(5-methyl-2-pyridin-4-yl-phenyl)-[4-oxidanyl-4-(phenylmethyl)piperidin-1-yl]methanone 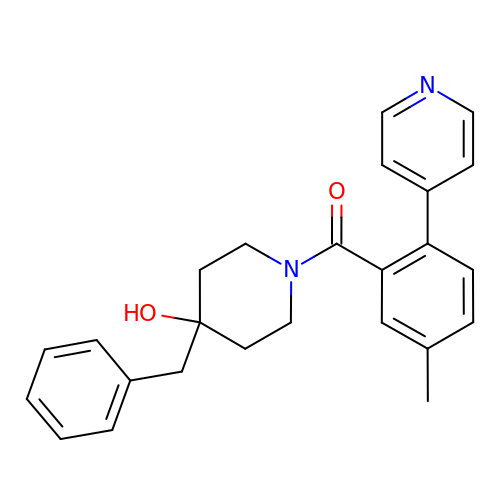| C25 H26 N2 O2 | SUPCEIFGZKXNGG-UHFFFAOYSA-N>[2x]KPGAPWWKSAVFYQVYPRSFKDTNGDGIGDFKGLTEKLDYLKGLGIDAIWINPHYASPNTDNGYDISDYREVMKEYGTMEDFDRLMAELKKRGMRLMVDVVINHSSDQHEWFKSSRASKDNPYRDYYFWRDGKDGHEPNNYPSFFGGSAWEKDPVTGQYYLHYFGRQQPDLNWDTPKLREELYAMLRFWLDKGVSGMRFATVATYSKTPGFPDLTPEQMKNFAEAYTQGPNLHRYLQEMHEKVFDHYDAVTAGEIFGAPLNQVP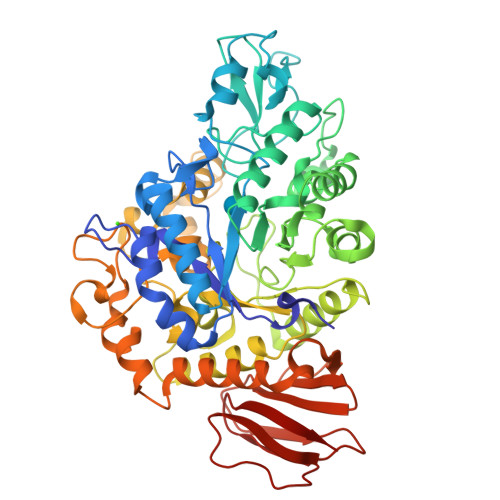LFIDSRRKELDMAFTFDLIRYDRALDRWHTIPRTLADFRQTIDKVDAIAGEYGWNTFFLGNHDNPRAVSHFGDDRPQWREASAKALATVTLTQRGTPFIFQGDELGMTNYPFKTLQDFDDIEVKGFFQDYVETGKATAEELLTNVALTSRNNARTPFQWDDSANAGFTTGKPWLKVNPNYTEINAAREIGDPKSVYSFYRNLISIRHETPALSTGSYRDIDPSNADVYAYTRSQDGETYLVVVNFKAEPRSFTLPDGMHIAETLIESSSPAAPAAGAASLELQPWQSGIYKVK>[2x]MVGYSSKLIFVSMITRHGDRAPFANIENANYSWGTELSELTPIGMNQEYNLGLQLRKRYIDKFGLLPEHYVDQSIYVLSSHTNRTVVSAQSLLMGLYPAGTGPLIGDGDPAIKDRFQPIPIMTLSA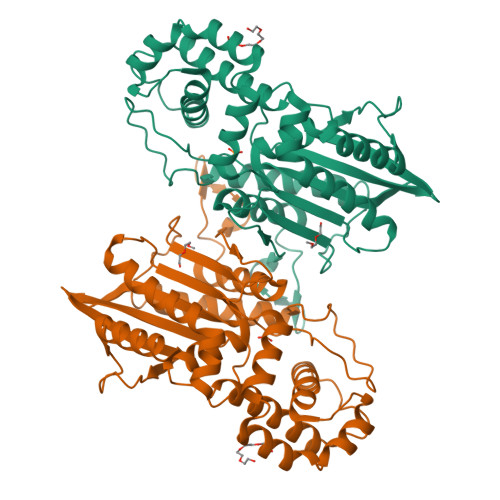DSRLIQFPYEQYLAVLKKYVYNSPEWQNKTKEAAPNFAKWQQILGNRISGLNDVITVGDVLIVAQAHGKPLPKGLSQEDADQIIALTDWGLAQQFKSQKVSYIMGGKLTNRMIEDLNNAVNGKSKYKMTYYSGHDLTLLEVMGTLGVPLDTAPGYASNLEMELYKDGDIYTVKLRYNGKYVKLPIMDKNNSCSLDALNKYMQSINEKFQKHHHHHH>GPMA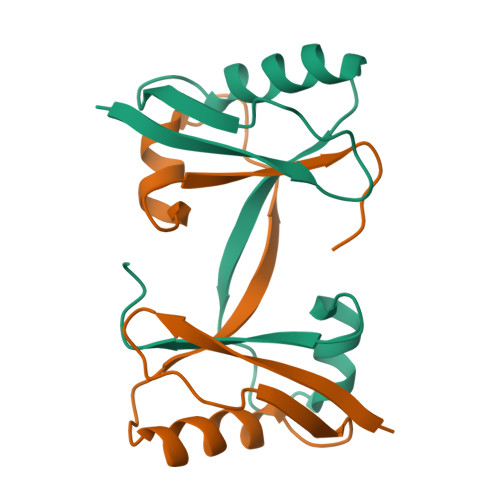TESPNSVQKIVVHLRATGGAPILKQSKFKVSGSDKFANVIDFLRRQLHSDSLFVYVNSAFSPNPDESVIDLYNNFGFDGKLVVNYACSMAWG[2x]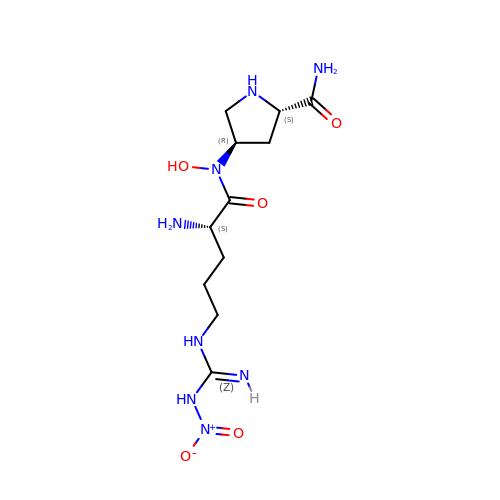(4R)-4-(HYDROXY{N~5~-[IMINO(NITROAMINO)METHYL]-L-ORNITHYL}AMINO)-L-PROLINAMIDE | C11 H22 N8 O5 | CTHMJCQUZVLLJU-CSMHCCOUSA-N> XDKTLEEIARELLKLA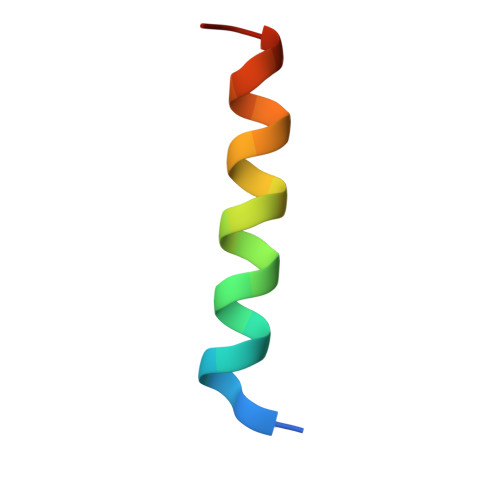LEIDKEIX> GAACGA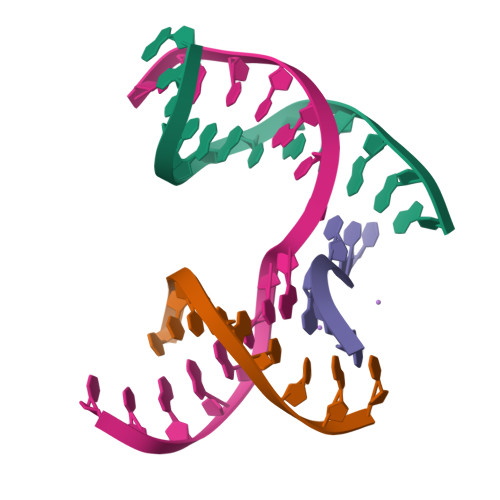CAGAGA;> CGTCGACTC;> TCTACG;> TCGAGTCGCTGTCGT The mono-ubiquitination of the histone protein H2B (H2Bub1) is a highly conserved histone post-translational modification that plays critical roles in many fundamental processes. In the budding yeast, the H2Bub1 reaction is catalyzed by the E3 enzyme Bre1 together with the E2 enzyme Rad6. In addition to the RING domain, Bre1 contains a N-terminal Rad6-binding domain (RBD) that also makes important contributions to the H2Bub1 catalysis. We found that the interaction stimulates Rad6’s enzymatic activity by allosterically increasing its active site accessibility and likely contribute to the H2Bub1 catalysis through additional mechanisms.

We screened through several fungal species and were able to crystallize the Kluyveromyces lactis Rad6 (KlRad6) in complex with the Kluyveromyces lactis Bre1 (KlBre1) N-terminal fragment 1-206 or 1-184 (crystal forms 1 and 2, respectively). The structures were refined to resolutions of 3.2 and 3.05 Å. The structures indicate that two KlBre1 N-terminal polypeptides dimerize to form an elongated RBD that binds to one KlRad6 molecule. Our structure indicates that KlRad6 interacts with the N-terminal region of KlBre1 RBD polypeptide 1 and N- and C-terminal regions of KlBre1 RBD polypeptide 2, which come together to form a single Rad6-binding site at one end of the RBD. It interacts with the back side of KlRad6 opposite from its active site, composed of strands β1–β3, the C-terminus of α4 and neighboring loops. The interface buries 2000 Å2 of surface area and contains hydrophobic, salt bridge and hydrogen bonding interactions. When the three KlRad6 molecules not mediating extensive crystal packing interactions in our structures are compared, large structural differences are observed for residues 90–98 and 115–121 surrounding KlRad6’s active site. The 90–98 region can be resolved in the electron density map in crystal form 1 but is mostly disordered in KlRad6 molecule 2 in crystal form 2, the equivalent Cα atoms in the 115–121 region are located as far as 5.2 Å apart. The temperature factors of these regions are also elevated in this structure, but less significantly. Together, these data indicate an increased mobility of regions 90–98 and 115–121 in KlRad6 in the KlBre1 RBD–Rad6 complex, suggesting that KlBre1 RBD allosterically increase the mobility of these regions.

>GSHMSTPARRRLMRDFKRMKEDSPPGVSASPLPDNVMIWNAMIIGPADTPYEDGTFRLLLEFDEEYPNKPPHVKFLSEMFHPNVYANGEICLDILQNRWTPTYDVASILTSIQSLFNDPNPASPANVEAATLFQDHKSQYVKRVKETVEKSWEDDMEDMADEDEDEE[2x];>[4x]MNDHFVKRPKLELSDPSEPLTQKDVIAFQKEALFRCLNKWRVKANQLVEENEVLAAGLSKTTESVSGCCSSIVVLARSVVEDCSDEQDKRFLQQLINTEDEHTLTQIISNNSARICELILKTSGSNISDNIGRLQELESLTLTLQKLLKSSENKLKKATEYYENIIAQYDRQDSESVSRVFNTADDDSNVKKEKQSSTGASSVNDE>GMLFDTSPKDNRKDFFDREKEIEKLKGLRAPITLVLGLRRTGKSSIIKIGINELNLPYIYLDLRKFEERNYISYKDFLLELQKEINKLVKRLPSLLKALKNIQGIVIMGNEIKFNWNRKDRLSFANLLESFEQASKDNVIIVLDEAQELVKLRGVNLLPALAYAYDNLKRIKFIMSGSEMGLLYDYLRVEDPESPLFGRAFSTVELKPFSREEAIEFLRRGFQEADIDFKDYEVVYEKIGGIP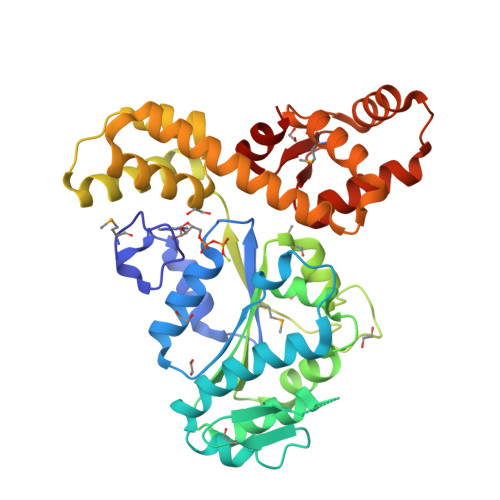GWLTYFGFIYLDNKNLDFAINQTLEYAKKLILKEFENFLHGREIARKRYLNIMRTLSKCGKWSDVKRALELEEGIEISDSEIYNYLTQLTKHSWIIKEGEKYCPSEPLISLAFS[2x]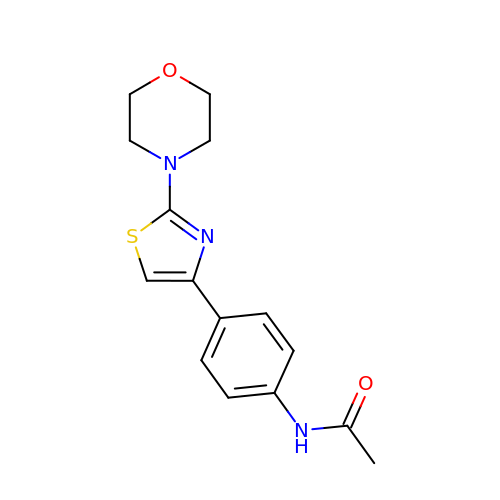N-[4-(2-morpholin-4-yl-1,3-thiazol-4-yl)phenyl]ethanamide | C15 H17 N3 O2 S | IUDYOCYEYLDKDX-UHFFFAOYSA-N> DTLCGSCGGNYTNDEFWICCDVCERWYHG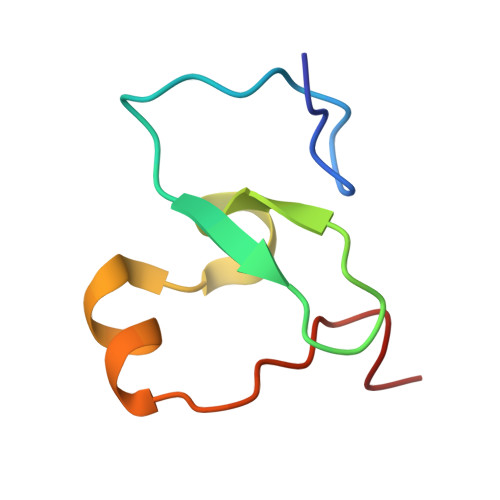KCVKITPAKAESIKQYKCPSCCT>[2x]MNKYTIAIDLGYGQIKGINQDNKRVIFPSIISSGKDRSLDTFFNSIDNIVDNIHVKILDEYFNEKEYFVGELAKRQPSNSSFINRDNKINSEENKVLLATALGLLIPNDLPNDTKIHIVTGLPLEHFIKQKQALNDMLKDFEHTIKFVDHNFSRNIKFEESNITLFPQGAGAIFSKINNDISSLLIKETFIGLIDVGFKTTDIVVFRINKDKEPVFEQEMSATLDGLGMINIYNTMDKAFTDNSRDGSKLNTEQLMLLCEEGKIFFKGDYIDLKKDLIKARKTLSTNIINKADGLWGSRKNSFNSIMIAGGGGKVLYNHLKLIEPNMCQLIDNPEFANAIGYLEFGKQF

Functional ParMRC plasmid segregation systems comprise an actin-like polymerizing motor (ParM), a centromere-like specific DNA sequence (parC), and an adaptor protein (ParR), which attaches a plasmid, via the parC, to each end of the growing ParM filament or filament bundle. Thus, the force generated from ParM polymerization is harnessed for plasmid segregation. Here we investigated the ParMRC cassette from pCBH, a 257 kb plasmid that carries the botulinum neurotoxin type B. This ParMRC cassette is also found on other C. botulinum plasmids, such as pCLK (267 kb) and pRSJ2_3 (245 kb), which encode neurotoxin types A and F, respectively. Despite the similarities to actin, pCBH ParM is a genuine ParM, since it has a closed β-barrel, a feature that is missing from actin and MreB structures.

Within each cross-section, an intermediate layer consisting of six hexagonal protomers showed the best local resolution. Inter-strand averaging for this intermediate layer led to a 4.2 Å map for the protofilament. The major difference between the monomer and filament protomers was the folding of a disordered region into a helix in F-ParM (F helix). The nucleotide-binding site in the pCBH G-ParM and F-ParM structures contain ADP and the magnesium ion is coordinated by Asp9, Asp195, and Gln168 equivalent to Asp11, Asp154, and Gln137 in actin, suggesting a common mechanism of ATP hydrolysis in which Gln168 (Gln137) directs the hydrolytic water towards the ATP γ-phosphate for nucleophilic attack. Next, we examined the pCBH ParM filament structure to understand how a single protomer forms strands of different lengths and twists. Firstly, the central interaction region involves long-chain charged and polar residues between subdomains 2 and 4 from the lower protomer and subdomain 3 from the upper protomer. Secondly, hydrophobic residues on the F helix from the subdomain 2 of the lower protomer fit into the hydrophobic pocket between subdomains 1 and 3 of the upper protomer. The hydrophobic residues in this interaction have fewer rotatable bonds than in the central interaction site. This architecture allows the hydrophobic interaction region to act like a ball-and-socket while the central interaction region is elastic due to the flexible long-chain interactions. The linker residues on either side of the F-helix are relatively flexible, which adds further pliancy into the intra-strand contacts.> QTARK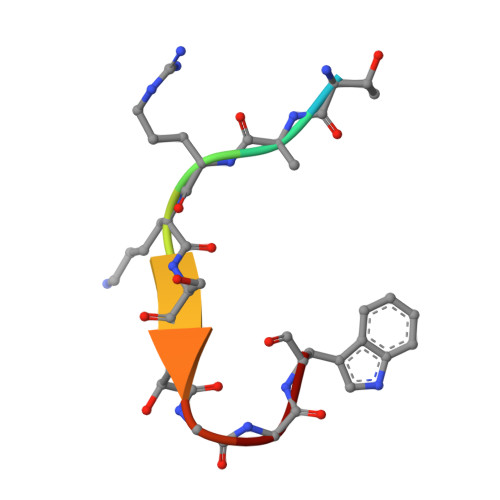STGGW> MGTLTIDGKNKILA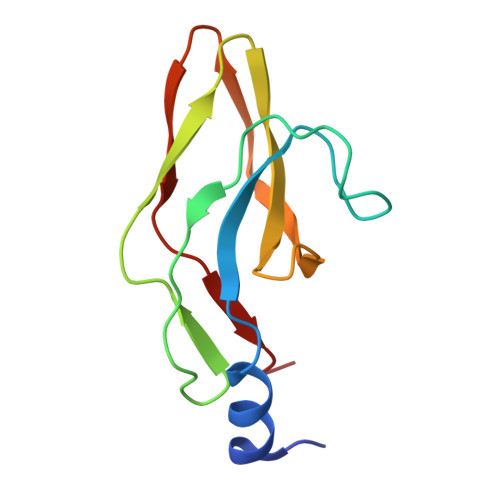TLTPTTIVLHNVDPTADPTANKVTQPVAIFFSEPNNGLIASEDTVNITVPASATVSHFSLWDDNSKCVATGALSSPQFFAEEGIYVISSVSIDLNK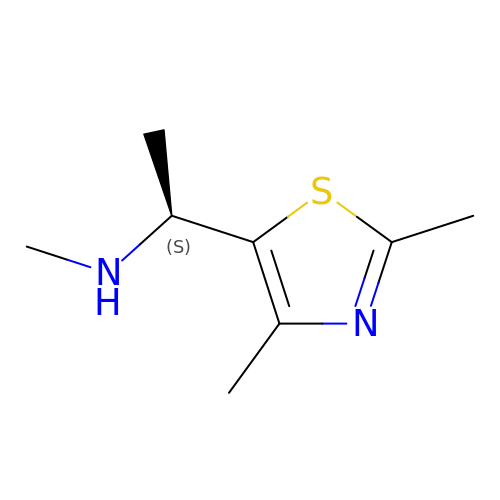(1S)-1-(2,4-dimethyl-1,3-thiazol-5-yl)-N-methylethan-1-amine | C8 H14 N2 S | YVLIGMQLZXNHQN-YFKPBYRVSA-N> QFAKPEDAVKYRQSALTLMASHFGRMTPVVKGQAPYDAAQIKANVEVLKTLSALPWAAFGPGTEGGDARPEIWSDAASFKQKQQAFQDNIVKLSAAAD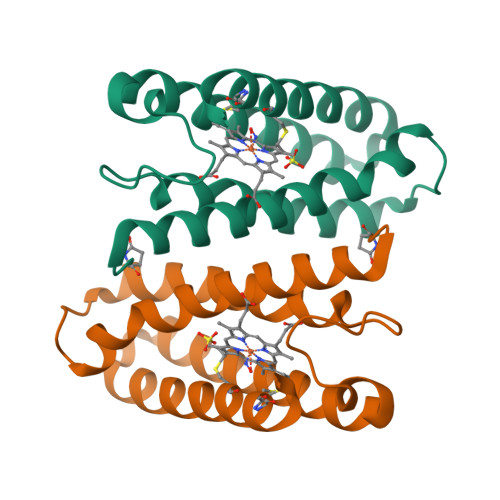AGDLDKLRAAFGDVGASCKACHQAYRKKK> MHHHHHHMLSVDDCFGMGRSAYNEGDYYHTVLWMEQVLKQLDAGEEATTTKSQVLDY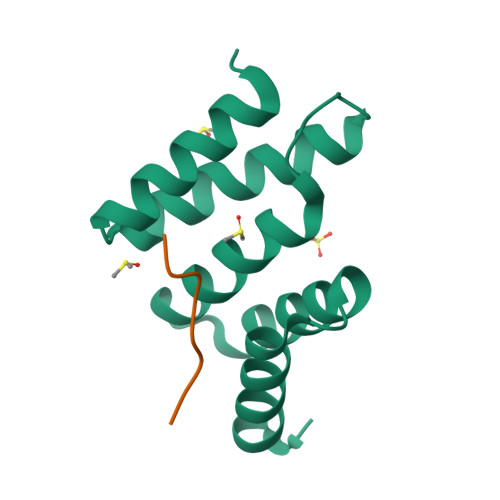LSYAVFQLGDLHRALELTRRLLSLDPSHERAGGNLRYFEQLLEEE;> PPGPEGPPG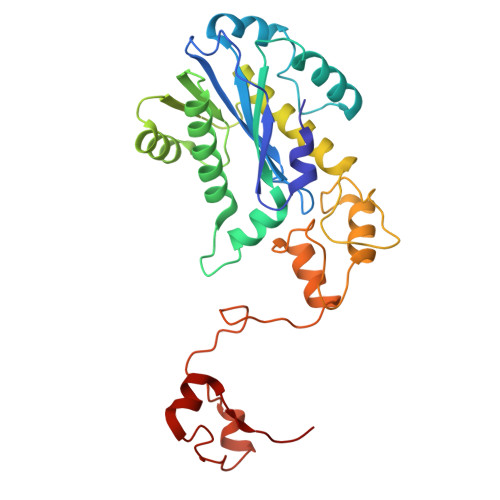> MDLSELERDNTGRCRLSSPVPAVCRKEPCVLGVDEAGRGPVLGPMVYAICYCPLPRLADLEALKVADSKTLLESERERLFAKMEDTDFVGWALDVLSPNLISTSMLGRVKYNLNSLSHDTATGLIQYALDQGVNVTQVFVDTVGMPETYQARLQQSFPGIEVTVKAKADALYPVVSAASICAKVARDQAVKKWQFVEKLQDLDTDYGSGYPNDPKTKAWLKEHVEPVFGFPQFVRFSWRTAQTILEKEAEDVIWEDSASENQEGLRKITSYFLNEGSQARPRSSHRYFLERGLESATSL> GSHMEATKRYLCLYLKESQEKFISNWKKRILV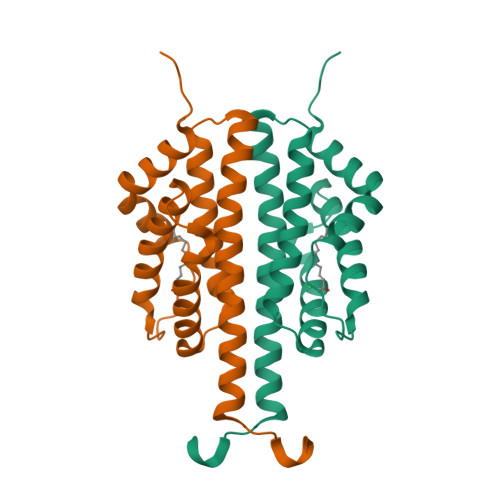HEHDPYKNEIIKNGTHLLHVFTMYMREEINLQDIEDISKKIAQERMDAKVNIADFIYNTNEGKKEILNTLFLLNPTGQECKVVIEQINLFFDHLIYSTIYSYYKLKKEYIHSYYELKKKYN>[2x]MEEVTNVMEYEAIAKKKLPKMVFDYYASGAEDQWTLAENRNAFSRILFRPRILIDVSKIDMSTTVLGFKISMPIMIAPTAMQKMAHPEGEYATARAASAAGTIMTLSSWATSSVEEVASTGPGIRFFQLYVYKDRNVVAQLVRRAERAGFKAIALTVDTPRLGRREADIKNRFVLPPFLTLKNF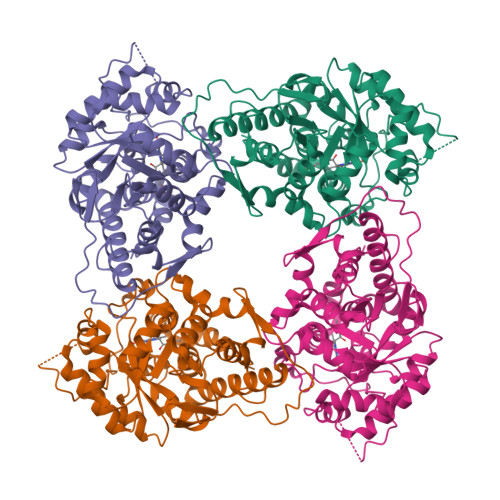EGLDLGKMDQASDSGLASYVAGQIDRTLSWKDVQWLQTITSLPILVKGVLTAEDARLAVQAGAAGIIVSNHGARQLDYVPSTIMALEEVVKAAQGRIPVFLDGGVRRGTDVFKALALGASGIFIGRPVVFSLAAEGEAGIKKVLQMLRDEFELTMALSGCRSLNEITRNHIVTEWDAPRAALPAPRL>[14x]MDHSITASYYDTTQQLSLLK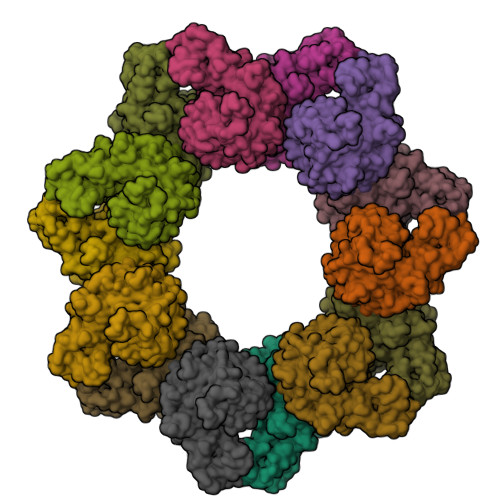HVLSEDKRPIAFIIAAGCPVSIRHNDAPLIPDVAGLTRKISDSFGGNPDSLLMKIIQNLKTTIPNPTIEDILSYIRLLQQIPMSGKIHDVENSVINALEESICELIEEEVNVDLPGNATPYHKIAAWINSINREHQVEIFTTNYDLLMEQALEELNVPYFDGFVGSKRAFFDIRTIEENKLPSRWSKLWKLHGSINWQLDKQTQTIWRGTPSKGCSLIHPSHLKYDQSRKMPYLVMMDQLKLFLNQPSAILITCGYSYKDQHINEVLSQGLQTNPNALIYGLQYDVLENYQEAKDMALKRSNLILLAKDRAIIGKKEGEWKPDPQSSQDNDPLLFFKLGDFQHLASFLEEISQYDWSKQND> MLRRTFAVVQKGERGLYFPINHRIVDRRIASGVTVEEADVQSRYRRELRTSFATGETRQTIPPAWSACERPTHFLSLRLPVRNVLRTRVNEMHNQILFSHQQHAPLLVPLEKLHITLGVMAISEREETERLASIYDCVSEVFSVIHPLQLRFRGLGTFGFGRVLFIRVVPEADFGILETAVSKIRRRVGGELKVDMKGNPHDSYVPHVTIAKIRSKQQTQFGSKIPISMWVEYQHHDFGDVTFSQVDICSMRGSKD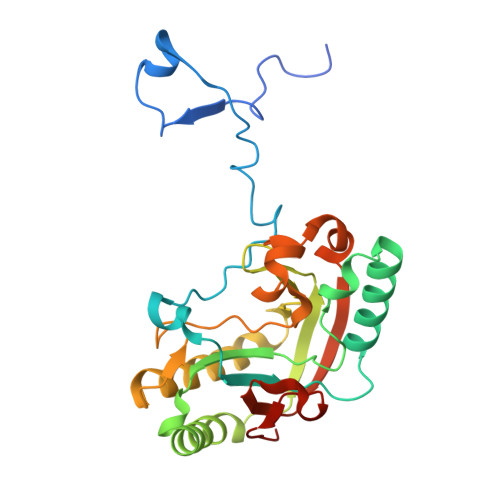GYYHTEGSVHLL>MAGGLSQLVAYGAQDVYLTGNPQITFFKTVYRRYTNFAIESIQQTINGSVGFGNKVSTQISRNGDLITDIVVEFVLTKGGNGGTTYYPAEELLQDVELEIGGQRIDKHYNDWFRTYDALFRMNDDRYNYRRMTDWVNNELVGAQKRFYVPLIFFFNQTPGLALPLIALQYHEVKLYFTLASQVQGVNYNGSSAIAGAAQPTMSVWVDYIFLDTQERTRFAQLPHEYLIEQLQFTGSETATPSATTQASQNIRLNFNHPTKYLAWNFNNPTNYGQYTALANIPGACSGAGTAAATVTTPDYGNTGTYNEQLAVLDSAKIQLNGQDRFATRKGSYFNKVQPYQSIGGVTPAGVYLYSFALKPAGRQPSGTCNFSRIDNATLSLTYKTCSIDA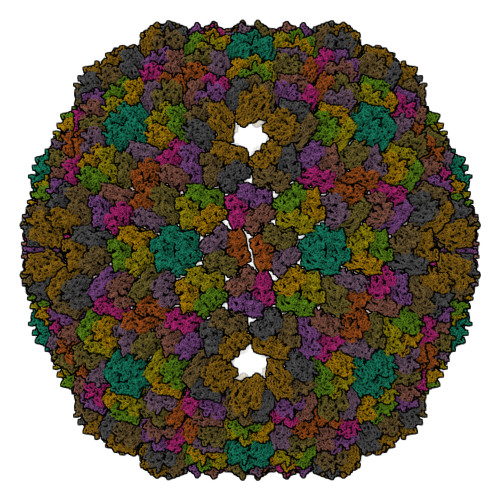TSPAAVLGNTETVTANTATLLTALNIYAKNYNVLRIMSGMGGLAYAN[13x]> MEVNDKAPAQARPTVFRWTGGGKEVYLSGS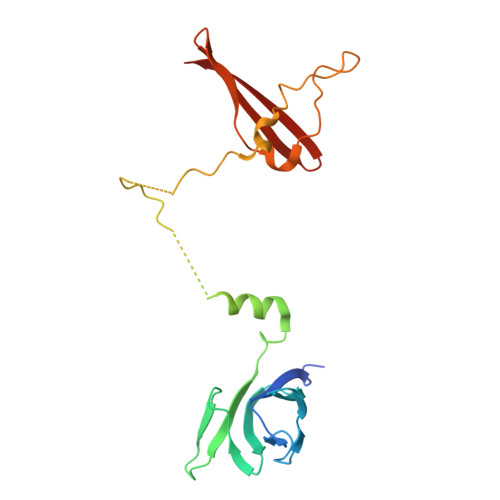FNNWSKLPLTRDHNNFVAILDLPEGEHQYKFFVDGQWTHDPSEPIVTSQLGTVNNIIQVKKTDFEVFDALMVDSQKCSDVSELSSSPPGPYHQEPYVCKPEERFRAPPILPPHLLQVILNKDTGISCDPALLPEPNHVMLNHLYALSIKDGVMVLSATHRYKKKYVTTLLYKPI> MKHHHHHHMKQNSPLDEENLTQENQDRGTHVDRGLASANVDFAFSLYKQLVLKAPDKNVIFSPLSISTALAFLSLGAHNTTLTEILKGLKFNLTETSEAEIHQSFQHLLRTLNQSSDELQLSMGNAMFVKEQLSLLDRFTEDAKRLYGSEAFATDFQDSAAAKK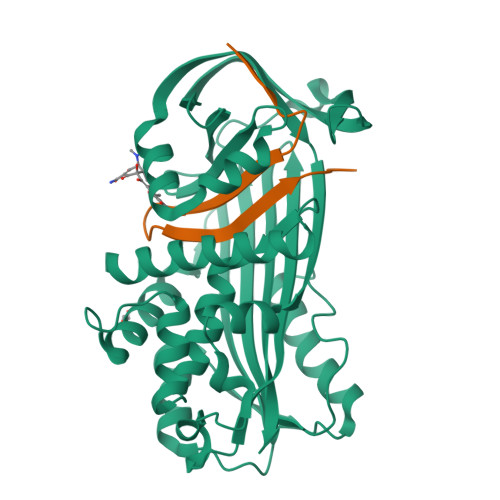LINDYVKNGTRGKITDLIKDLDSQTMMVLVNYIFFKAKFEMPFDPQDTHQSRFYLSKKKYVMVPMMSLHHLTIPYFRDEELSCTVVQLNYTGNASALFILPDQDKMEEVEAMLSQETLARFFDSLEFREIGELYLPKFSISRDYNLNDILLQLGIEEAFTSKADLSGITGARNLAVSQVVHKAVLDVFEEGTEASAATALEVLFQ;> GPLVETRTIVRFNRPFLMIIVDHFTWSIFFMSKVTNPKQA2-{[(3-bromophenyl)methyl]amino}-5-methyl[1,2,4]triazolo[1,5-a]pyrimidin-7(6H)-one | C13 H12 Br N5 O | 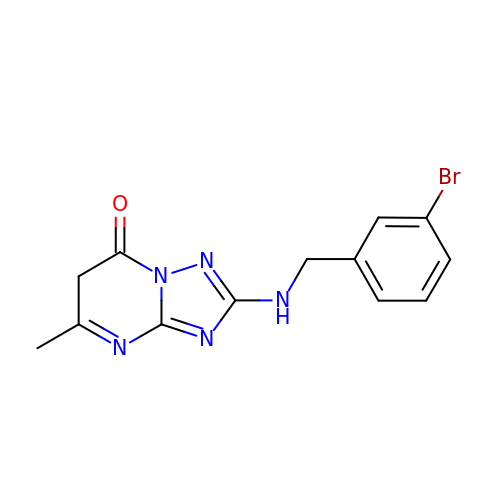NONMKRIVUVFGSW-UHFFFAOYSA-N>[42x]HEFAELFYRTYIVTPDQAGFQLSIRRNLVWEGWTGEGLSGEKQEISKRNILQGLLDYTTLETNSTELIPVIQSGENDEQFIDPSVLPAQTVKQGKDTFDTNFLKFSENGEGFNLLMLAQTPSRLKKGSMTFTDSLDSRIALKQLLISVTKGGTTELFALDVNRDQYAAYTATREYNFRLMQLKFHTSLGLGEESTTVAGAESALLKDLFDLGYRIELDVKVDGEMNVENGNGDTSLRALRLARVFDKEGKEIALTDSRVSAALSGLTVTGVGYSLEARLTNINQLEMGLLIDSDVQKQGFMIPTLPPLVIVKPAMVEDDKTYPRLEALTTAYRIQQMRNNAVTTLLNRADTLKSYLGVGVPHPIESNLGLEGVGQYYVRPYYNEATIDVLNDLNNLTSAAKQTDIQGLIVSKINEMVYTADQLTGYTAALEAAFSGRSPKPHVAIGTDMRLPQY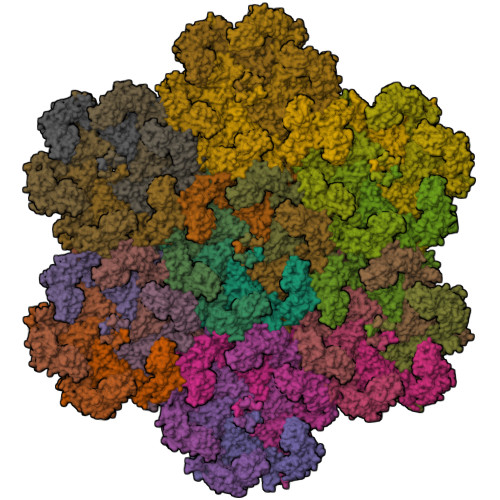IQINGDDRTVGIGYDYTIARISDLRMKDKIVMTFILPNESEPHPLQHGVLGFIPEYLVDFNMIRNQRIGREIRLTPRYRYFNFLPIMLVINVINLEEAIAQRTALDVNETQVTPAS>MAASKKAVLGPLVGAVDQGTSSTRFLVFNSKTAELLSHHQVEIEQKFPKEGWVEQDPKEILQSVYECIEKTCEKLGQLNIDISNIKAIGVSNQRETTVVWDKLTGEPLYNAVVWLDLRTQSTVANLSKIIPVNNNFVKTKTGLPLSTYFSAVKLRWLLDNVRKIQKAVEEDRALFGTIDSWLIWSLTGGARGGVHCTDVTNASRTMLFNIHSLEWDKELCEFFEVPMKILPNVRSSSEIYGLMKAGALEGVPISGCLGDQSAALVGQMCFQDGQAKNTYGTGCFLLCNTGHKCSVAIAGAVVRWLRDNLGIIKTSEEIEKLAKEVGTSYGCYFVPAFSGLYAPYWEPSARGIICGLTQFTNKCHIAFAALEAVCFQTREILDAMNRDCGIPLSHLQVDGGMTNNKILMQLQADILYIPVVKPSMPETTALGAAMAAGAAEGVGVWSLKPEDLSAVTMERFEPQINAKESEIRYSTWKKAVKKSMGWV[4x];>MASYGQTCPRPMCIPPSYADLGKAARDIFNKGFGFGLVKLDVKTKSCSGVEFSTSGSSNTDTGKVTGTLETKYKWCEYGLTFTEKWNTDNTLGTEIAIEDQICQGLKLTFDTTFSPNTGKKSGKIKSSYKRECVNLGCDVDFDFAGPAIHGSAVFGYEGWLAGYQMTFDSAKSKLTRNNFAVGYRTGDFQLHTNVNDGTEFGGSIYQKVCEDLDTSVNLAWTSGTNCTRFGIAAKYQLDPTASISAKVNNSSLIG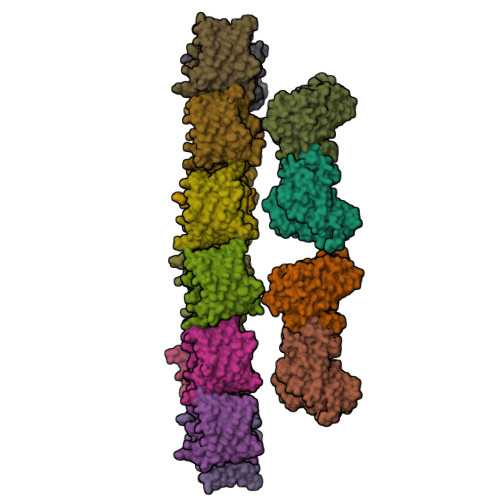VGYTQTLRPGVKLTLSALVDGKSINAGGHKLGLALELEA[12x]>[2x]ANADNYKNVINRTGAPQYMKDYDYDDHQRFNPFFDLGAWHGHLLPDGPNTMGGFPGVALLTEEYINFMASNFDRLTVWQDGKKVDFTLEAYSIPGALVQKLTAKDVQVEMTLRFATPRTSLLETKITSNKPLDLVWDGELLEKLEAKEGKPLSDKTIAGEYPDYQRKISATRDGLKVTFGKVRATWDLLTSGESEYQVHKSLPVQTEINGNRFTSKAHINGSTTLYTTYSHLLTAQEVSKEQMQIRDILARPAFYLTASQQRWEEYLKKGLTNPDATPEQTRVAVKAIETLNGNWRS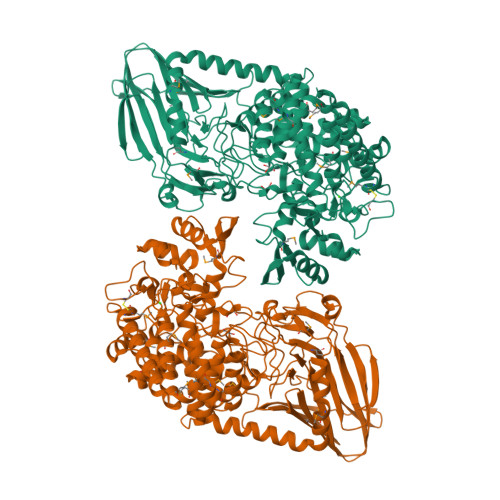PGGAVKFNTVTPSVTGRWFSGNQTWPWDTWKQAFAMAHFNPDIAKENIRAVFSWQIQPGDSVRPQDVGFVPDLIAWNLSPERGGDGGNWNERNTKPSLAAWSVMEVYNVTQDKTWVAEMYPKLVAYHDWWLRNRDHNGNGVPEYGATRDKAHNTESGEMLFTVKKGDKEETQSGLNNYARVVEKGQYDSLEIPAQVAASWESGRDDAAVFGFIDKEQLDKYVANGGKRSDWTVKFAENRSQDGTLLGYSLLQESVDQASYMYSDNHYLAEMATILGKPEEAKRYRQLAQQLADYINTCMFDPTTQFYYDVRIEDKPLANGCAGKPIVERGKGPEGWSPLFNGAATQANADAVVKVMLDPKEFNTFVPLGTAALTNPAFGADIYWRGRVWVDQFWFGLKGMERYGYRDDALKLADTFFRHAKGLTADGPIQENYNPLTGAQQGAPNFSWSAAHLYMLYNDFFRKQ>[6x]AATHTGPTPADAVPAYPFSLPHALDLDPHYAELRRDEPVSRVRLPYGEGTAWLVTRMSDARIVLGDSRFSTAAATDPATPRMFPTPPEPDGVLAQDPPDHTRLRRLVGKAFTARRVEEMRP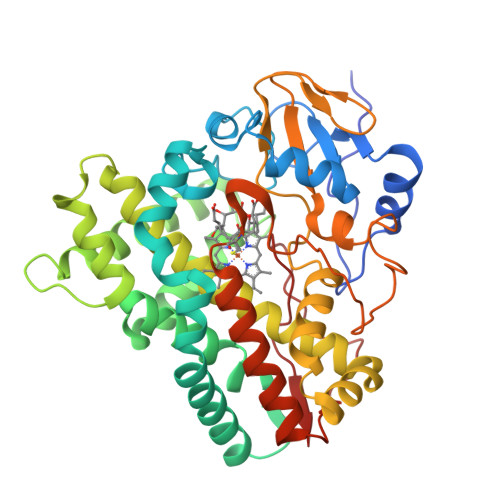RVRSLVDSLLDDMVAHGSPADLVEFLAVPFPVAVICELLGVPLEDRDLFRTFSDAMLSSTRLTAAEIQRVQQDFMVYMDGLVAQRRDAPTEDLLGALALATDNDDHLTKGEIVNMGVYLLIAGHETSVNQITNLVHLLLTERKRYESLVADPALVPAAVEEMLRYTPLVSAGSFVRVATEDVELSTVTVRAGEPCVVHFASANRDEEVFDHADELDFHRERNPHIAFGHGAHHCIGAQLGRLELQEALSALVRRFPTLDLAEPVAGLKWKQGMLIRGLERQIVSW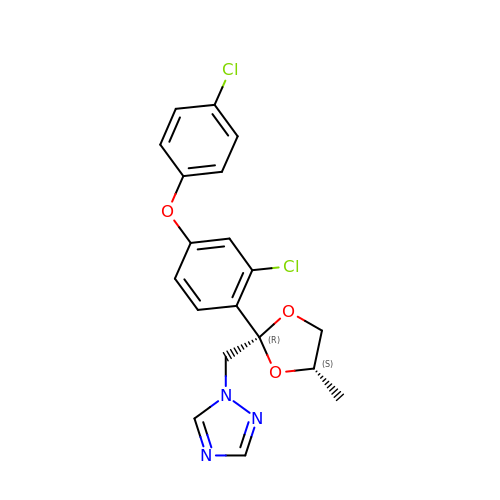1-[[(2~{R},4~{S})-2-[2-chloranyl-4-(4-chloranylphenoxy)phenyl]-4-methyl-1,3-dioxolan-2-yl]methyl]-1,2,4-triazole | C19 H17 Cl2 N3 O3 | BQYJATMQXGBDHF-DJJJIMSYSA-N> GPAMSPESKNAVQMQSEKSASDSGEVATEKAPAKQDTKEKSGTETEKGKEDGTKGTKDSSADKETSAEASEKGTVVTETADDDLFTTYRLDLEDARSKEREELNAIVSSDDATAKEKSEAYDKMTALSEVEGTEKQLETLIKTQGYEDALVNAEGDKINITVKSDKHSKSKATAIIDLVAKEIKTMKDVAVTFEPSK;> GPAMQSVSNDEVKDQLADNGGNSAYDNNDDAVEVGK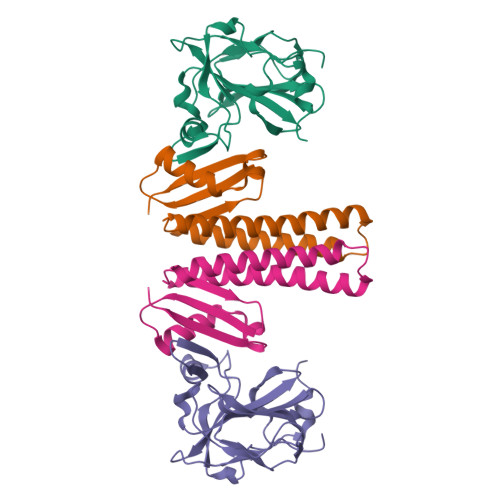SMENVAMPVVDSENVSVVKKFYETDAAKEEKEAALVTYNNTYSLSKGIDLAEKDGKDFDVSASLSGTVVKAEKDPVLGYVVEVEHADGLSTVYQSLSEVSVEQGDKVKQNQVIGKSGKNLYSEDSGNHVHFEIRKDGVAMNPLNFMDKPVSSIEKAATQETEESIQQSSEKKDGSTEKGTEEKSGEKKDDSTDKSGSKESSTTEDTEQS> ARHVLLQAEFYQRSEGPDKAWAQFGFHFDADELFHVELDAAQTVWRLPEFGRFASFEAQGALQNMA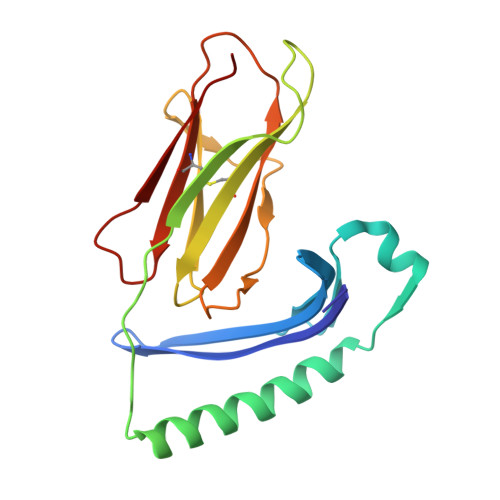VGKQNLEVMISNSNRSQQDFVTPELALFPAEAVSLEEPNVLICYADKFWPPVATMEWRRNGAVVSEGVYDSVYYGRPDLLFRKFSYLPFVPQRGDVYSCAVRHWGAEGPVQRMWEPE>NLYFQSMRILVTGGSGLVGKAIQKVVADGAGLPGEDWVFVSSKDADLTDTAQTRALFEKVQPTHVIHLAAMVGGLFRNIKYNLDFWRKNVHMNDNVLHSAFEVGARKVVSCLSTCIFPDKTTYPIDETMIHNGPPHNSNFGYSYAKRMIDVQNRAYFQQYGCTFTAVIPTNVFGPHDNFNIEDGHVLPGLIHKVHLAKSSGSALTVWGTGNPRRQFIYSLDLAQLFIWVLREYNEVEPIILSVGEEDEVSIKEAAEAVVEAMDFHGEVTF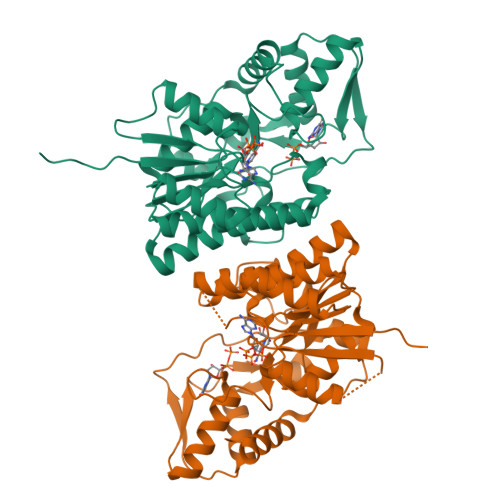DTTKSDGQFKKTASNSKLRTYLPDFRFTPFKQAVKETCAWFTDNYEQAR[2x]Here, we explore and test these notions using resurrected Precambrian β-lactamases11 as scaffolds for the engineering of completely new active sites. Of these systems, resurrected Precambrian β-lactamases have been thoroughly characterized in terms of their structure, function and stability. These putative ancestral proteins have been shown to be highly stable and able to efficiently degrade several antibiotics. A hydrophobic-to-ionizable amino acid replacement generates a buried (or partially buried) residue with the perturbed properties that are useful in catalysis and conformational flexibility assists the generation of a completely new active site by facilitating substrate and transition-state binding. We have shown that, when using resurrected Precambrian β-lactamases as scaffolds for protein engineering, a minimalist design approach based on this mechanism leads to levels of catalysis for the Kemp elimination reaction of up to approximately seven orders of magnitude above the rate of the uncatalysed reaction, as well as to significant ester hydrolysis activity.

In addition, we have also used here proteins encoded by alternative sequences at the GNCA node (common ancestor of Gram-negative bacteria). As is custormary in the field, these alternative sequences were derived from a random weighted sampling of the posterior probability distribution. They differ from the most probabilistic sequence at 8–20 positions. Second, the GNCA4 scaffold appears to be more rigid (in the new active site region) than the GNCAMP scaffold, despite the fact that GNCA4 leads to higher levels of Kemp elimination activity upon the W229D mutation. However, 3D-structure determination shows that the GNCA4 is actually more preorganized for transition-state binding than the GNCAMP scaffold. This can again ultimately be viewed as a reflection of flexibility at the GNCA node, as mutations removed from the active site can easily shift the conformational equilibria at this node. Clearly, the specific mutations present in the GNCA4 scaffold have led to the population of a conformation in the W229D variant with a cavity where the substrate can easily form a reactive conformation, and with better architecture for effective transition-state stabilization. Remarkably, however, the new active site behaves differently and engineered β-lactamases encoded by several alternative reconstructions at the GNCA node (common ancestor of Gram-negative bacteria) display Kemp elimination activities that span a ∼30-fold range. The several GNCA sequences studied differ among themselves at 8–20 positions, which are, in essentially all cases, distal from the neighbourhood of the Kemp elimination active site.

> MAAALSEQLAELEKRSGGRLGVAVLDTATGRRFGYRGDERFPMCSTFKALLAAAVLARVDQGKENLDRRITYGKEDLVDYSPVTEKHVGDGMTVAELCEAAITYSDNTAANLLLEALGGPAALTAFLRSIGDNVTRLDRWEPELNTAAPGDPRDTTTPAAMAATLRTLLLGDVLSPASRQQLVDWLIANKTGDKRLRAGLPADWRVGDKTGTGEHGTTNDIAVIWPPNRAPILVAVYLTESQVDADARDAVIAEVARLVVAAFHHHHHH> AKDFSGAELYTLEEVQYGKFEARMKMAAASGTVSSMFLYQNGSEIADGRPWVEVDIEVLGKNPGSFQSNIITGKAGAQKTSEKHHAVSPAADQAFHTYGLEWTPNYVRWTVDGQEV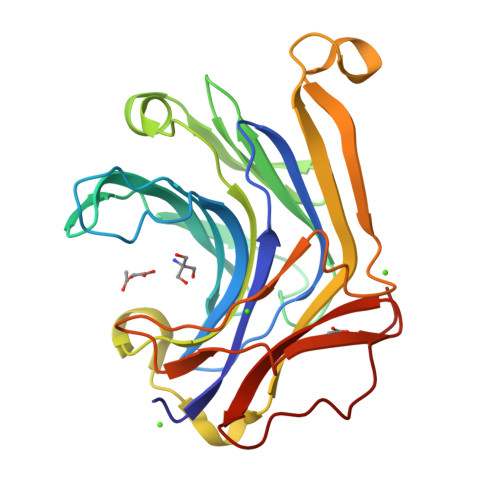RKTEGGQVSNLTGTQGLRFNLWSSESAAWVGQFDESKLPLFQFINWVKVYKYTPGQGEGGSDFTLDWTDNFDTFDGSRWGKGDFTFDGNRVDLTDKNIYSRDGMLILALTRKGQESFNGQVPRD>GHMSGQRWELALGRFWDYLRWVQTLSEQVQEELLSSQVTQELRALMDETMKELKAYKSELEEQLTPVAEETRARLSKELQAAQARLGADMEDVCGRLVQYR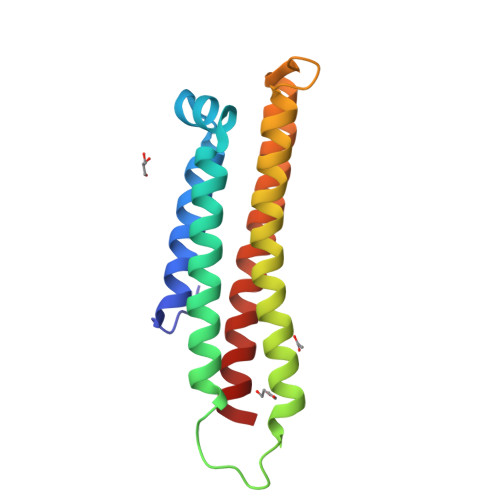GEVQAMLGQSTKELRNRLASHLGKLQDRLLRDADDLQKRLAVYQAG[2x]>[2x]MGSMRRVVGKRVQEFSDAEFEQLRS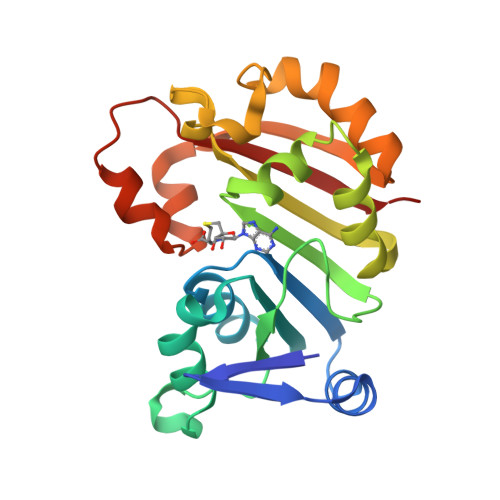QYDDVVLDVGTGDGKHPYKVARQNPSRLVVALDADKSRMEKISAKAAAKPAKGGLPNLLYLWATAERLPPLSGVGELHVLMPWGSLLRGVLGSSPEMLRGMAAVCRPGASFLVALNLHAWRPSVPEVGEHPEPTPDSADEWLAPRYAEAGWKLADCRYLEPEEVAGLETSWTRRLHSSRDRFDVLALTGTISP> ASVLWFQGGACSGNTMSFLNADEPNVVDLIVDFGLDLLWHPSLGLELGNNAQKVFWDCAKGERPLDIFVFEGTVIEAPNGTGQMDMFAGRPMKDWVTDLAGAAQIVVAIGDCACFGGIPAMEPNPSGSTGLQFHKREKGGFLGPDFRSKMGLPVINVPGCPA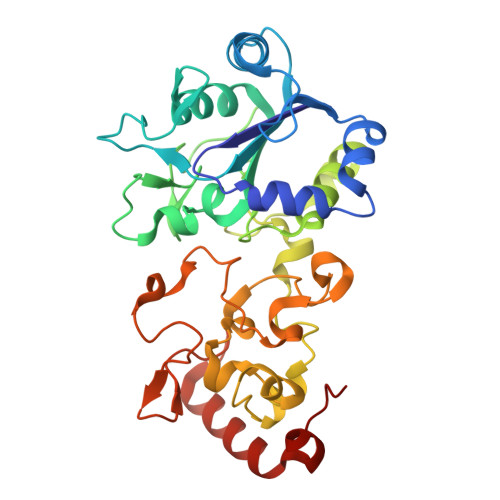HPDWITQILVALATGRAGDITLDDLHRPETFFKTFTQTGCTRVQFFEYKQSTLSFGEGTRTGCLFYEFGCRGPMTHSPCNRILWNRQSSKTRAGMPCLGCTEPEFPHFDLAPGTVFKTQKVSGMIPKEVPEGTDHLTYMGLAAAARIAAPQWSKEDMFVV One example is the sperm-specific SLC9C1 that belongs to the SLC9 superfamily of cation/proton antiporters, known as Na+/H+ exchangers (NHEs), which are essential for the regulation of intracellular pH, sodium homeostasis and cell volume. The transport domain (TD) is accompanied by a voltage-sensing domain (VSD) and a cyclic-nucleotide binding domain (CNBD), which are regulatory units usually found in voltage-gated cyclic-nucleotide-modulated ion channels, also referred to as CNBD ion channels. In a recent patch-clamp fluorimetry study, the functional integrity of the domains was confirmed for SLC9C1 from the sea urchin Strongylocentrotus purpuratus, termed SpSLC9C1, identifying it as a Na+/H+ exchanger that is activated strictly by hyperpolarization and modulated by cyclic nucleotides (cNMPs). Specifically, SpSLC9C1 adapted to mediate cellular alkalization in sperm only in response to chemoattractant-induced hyperpolarization.

A general observation, evident from the local resolution maps, is that in all of our SpSLC9C1 structures the protein displays substantial structural heterogeneity for most of its domains except for the TD, which indicates that it might be locked. Focused 3D classifications at the dimer level could not resolve the conformational flexibility, which suggests that the movements of the domains are, to a degree, independent within the dimer. Therefore, focused heterogeneity analysis at the protomer level with a mask excluding the TD was performed instead. For the apo dataset, four conformations with a resolution range of 3.2–3.4 Å and with substantially improved densities of all the domains could be distinguished. The most pronounced differences are confined to the region of the CHs. They are accompanied by subtle conformational transitions in the VSD and CNBD, which further indicates that the CHs might play a central role in coupling voltage sensing and cAMP modulation to exchange activity in the TD. In line with this assumption, the extended cytoplasmic region of S4 forms several interaction areas with CHs, which have to rearrange upon voltage activation.

> MSKKRVVKLRELVPAVAALAVAVLIQSATGSSGGSGHTPTTQATHADDHDLTTHNGTEEHDDGHDDGHDDLHAHAPKVIVFISGSCLFGAISRSLFKKLPIPYTVVLLILGAILGVVASNVPLVEEHTRDVAHMDPHVLLQIFLPVLIFESAFAMDVHTFMRSFSQVCILALFGLVVASVLTAVLAMNLFNYNWNFSEAMMFGAIMSATDPVAVVALLKDLGASKQLGTIIEGESLLNDGCAIVIFNVFMKMVFFPQLTSTVGQNVLYFLQVAVAGPLWGYAVAKVTVFFLSHIFNDALVEITITLAATYLTYYIGDIWLEVSGVLAVVVLGLIVNAEKTSISPEVEVFLHRFWEMLAYLANTLIFMMVGVVVTQKALVAVDKMDWFYLIILYLAITIIRGMVISLFSPILSRIGYGLTWRNAVIMTWGGLRGAVGLALALVVENLAGNDVIGSKFLFHTAGIVVLTLVINATTIQTLLRILGMSDISIPKRLAMAGAVRRIHEGQNRTLNMLKSDRFLADADWDIATAACEISDPYSALSDDENAPADELTLGERKSVCPGCKAMVPNEPSPREFADMMEEARLRMLKAEKISYWKQFEHGMLAREALRLLVQHAEVAADEKDQFILVDDLKKSWQIKGIYPWLKRKLEDLISEKKIAAIPMPKYKLGKLMYKICHHMAFEVTINIAIVLNIVPIIMEFVVQDKMASVSTMAAPGSTVSSEPSSSQKIEDALRISNYVFFVIYAIEAIVKILGLGRHYIVSHWNKFDAFILVVALVDIIIAETLLKGSITINLSSIKVVKLFRLLRGLRMLRLTKALIPKLILVVNGKINNQLSLGYDVGKGYIIGEEEVGKIIDRMVDNKKILRELKHISETGRLQVVKELGLLQREHPGIAVSVKTRQAIRTILNHSRETIHELQGAGLLDEMEAHKLELTVEIKMKRLMNAPSSIPPPPPENLLKNVSWLAGDMKLIDFIKARASLLHFDYGEVIVREGDESDGLFLIVSGLVKLYGKSAFLDHDNPPVTAGSEENEVFEDYLTVGNVIGEMGVLTKKPRNATVTCETTVQVYFITAEDMNIAIDTFTLYPSLEYRLWRVVAIRIATPLIMEQMAFQGWTQEKVKLHLERGYLVDLAESHFQFNIDATLEDVILINGTAYNAHTREEIRSPCLISRTVHKLTFQYTATEEPRLFVVRNAEYNGPILDGRLDVDSKRSLISITEISSNMCLKHAAELRQKNSKVMLSRKSSGAAAKEEEDCIPNTSDVEQAAGVSPSVPTKTTPKPKSFLPSLGLSMSKERVNGEAVEESPVKTKQGEETPETEEGAAPRVNVALEVLFQ>[10x]MSLINTKIKPFKNQAFKNGEFIEITEKDTEGRWSVFFFYPADFTFVCPTELGDVADHYEELQKLGVDVYAVSTDTHFTHKAWHSSSETIAKIKYAMIGDPTGALTRNFDNMREDEGLADRATFVVDPQGIIQAIEVTAEGIGRDASDLLRKIKAAQYVASHPGEVCPAKWKEGEATLAPSLDLVGKYFSKHN

The Prx subfamily enzyme Prx1, also typically called 2-Cys Prx, is among the most highly expressed, soluble proteins in the cell, and is characterized by two conserved cysteine residues. We used the mechanistically well understood E. coli as a prototype to construct a chimeric Prx, EcAhpC1-186-YFSKHN, composed of EcAhpC (residues 1–186) and the C-terminal YFSKHN-segment of human Prx 2, to be compared with wild-type (WT) EcAhpC. The chimeric EcAhpC1-186-YFSKHN described here demonstrates, that transformation of the human C-terminal YFSKHN-helix into the related bacterial AhpC confers sensitivity to over-oxidation on the chimeric enzyme. Structural details of the oxidized and reduced chimeric EcAhpC1-186-YFSKHN provide novel insights into sub-steps during the catalysis of peroxide reduction, enabling the transition from a fully folded to a locally unfolded conformation. Together with mutational and enzymatic studies these data unravel the fundamental role of the C-terminal tail as a molecular switch that mediates the structural transition between the FF and LU state during the catalytic cycle.

To understand the structural effect of the human YFSKHN-helix in general, in particular inside the chimeric EcAhpC1-186-YFSKHN, as well as to identify the individual amino acids essential for sensitivity to oxidative inactivation of Prxs, the crystal structure of oxidized EcAhpC1-186-YFSKHN has been solved at 2.7 Å resolution. The asymmetric unit contains one decamer composed of five catalytic dimers (α2)5 with each subunit containing one catalytic active peroxidatic and one resolving cysteine. The intermolecular disulphide bond observed between CP47 and CR166′ in the dimer interface confirms the oxidized state of the EcAhpC1-186-YFSKHN structure. The peroxidatic cysteine (CP47), located in the first turn of helix α2, adopts an LU conformation in the oxidized structure. In most of the disulphide bonded active sites of the decameric and oxidized EcAhpC1-186-YFSKHN, the C-terminal arm beyond the resolving cysteine (CR166) is disordered, indicating the high flexibility of the C-terminus. However, the structure in chain (H) could be resolved until residue 177, showing amino acids 167 to 177 oriented away from the active site and stacked against the neighboring symmetry molecule. Similarly, the C-termini of chains A, G and J are also stabilized by the packing interactions with the symmetry related molecules. The average main chain B-factors analysis revealed three dynamic regions of oxidized EcAhpC1-186-YFSKHN: (i) the CP47 containing α2-helix, (ii) helix α5 that contains residues S86 and T88, and (iii) the C-terminal tail region. The sulfate ions observed in the interface region of the structure, emphasis their role in stabilizing the oxidized AhpC in a decameric form in solution. Superposition of the recently resolved oxidized EcAhpC structure with the corresponding dimer of the oxidized EcAhpC1-186-YFSKHN one resulted in an r.m.s.d. value of 0.4 Å.>[2x]HHHHHHENLYFQGSMDALQLANSAFAVDLFKQLSEKEPLGNVLFSPIALSTSLSLAQVGAKGDTANEIGQVLHFENVKDVPFGFQTVTSDVNKLSSFYSLKLIKRLYVDKSLNLSTEFISSTKRPYAKELETVDFKDKLEETKGQINNSI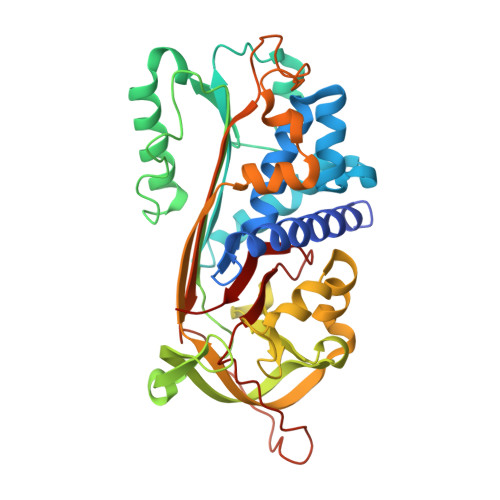KDLTDGHFENILADNSVNDQTKILVVNAAYFVGKWMKKFSESETKESPFRVNKTDTKPVQMMNMEATFSMGNIDSINSKIIELPFQNKHLSMFILLPKDVEDESTGLEKIEKQLNSESLSQWTNPSTMANAKVKLSIPKFKVEKMIDPKASLENLGLKHIFSEDTSDFSGMSETKGVALSNVIHKVSLEITEDGGDSIEVPGARILQHKDELNADHPFIYIIRHNKTRNIIFFGKFSSP>VVTLGYWDIRGLAHAIRLLLEYTETPYQERRYKAGPAPDFDPSDWTNEKEKLGLDFPNLPYLIDGDVKLTQSNAILRYIARKHNMCGETEVEKQRVDVLENHLMDLRMAFARLCYSPDFEKLKPAYLEQLPGKLRQLSRFLGSRSWFVGDKLTFVDFLAYDVLDQQRMFVP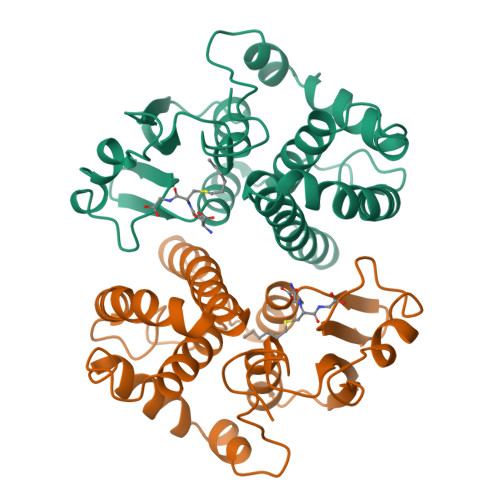DCPELQGNLSQFLQRFEALEKISAYMRSGRFMKAPIFWYTALWNNKKE[2x]>GPMGSKQMGSMHPVQVIAVTGGKGGVGKTNVSVNLALALADLGRRVMLLDAALGLANVDVLLGLTPKRTLADVIEGRCELRDVLLLGPGGVRIVPAASGTQSMVHLSPMQHAGLIQAFSDISDNLDVLVVDTAAGIGDSVVSFVRAAQEVLLVVCDEPTSITDAYALIKLLNRDHGMTRFRVLANMAHSPQEGRNLFAKLTKVTDRFLDVALQYVGVIPYDESVRKAVQKQRAVYEAFPRSKASLAFKAVAQKVDSWPLPANPRGHLEFFVERLVQHPATGSAV[2x];>MGSWRETKLLLIDDNLDRSRDLAVILNFLGEDQLTCNSEDWREVAAGLSNSREALCVLLGSVESKGGAVELLKQLASWDEYLPILLIGEPAPADWPEELRRRVLASLEMPPSYNKLLDSLHRAQVYREMYDQARERGRSREPNLFRSLVGTSRAIQQVRQMMQQVADTDASVLILGESGTGKEVVARNLHYHSKRREGPFVPVNCGAIPAELLESELFGHEKGAFTGAITSRAGRFELANGGTLFLDEIGDMPLPMQVKLLRVLQERTFERVGSNKTQNVDVRIIAATHKNLEKMIEDGTFREDLYY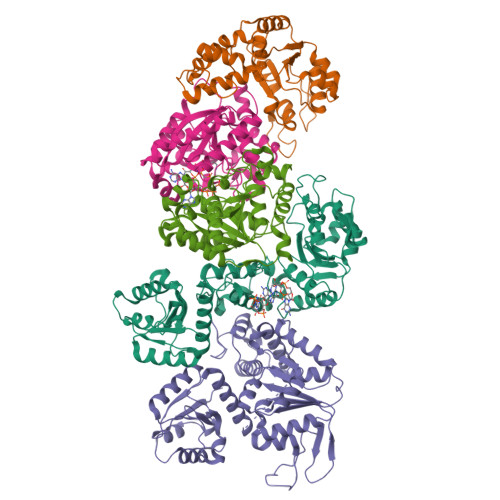RLNVFPIEMAPLRERVEDIALLLNELISRMEHEKRGSIRFNSAAIMSLCRHDWPGNVRELANLVERLAIMHPYGVIGVGELPKKFRHVD[3x]>SPILGYWKIKGLVQPTRLLLEYLEEKYEEHLYERDEGDKWRNKKFELGLEFPNLPYYIDGDVKLTQSMAIIRYIADKHNMLGGCPKERAEISMLEGAVLDIRYGVSRIAYSKDFETLKVDFLSKLPEMLKMFEDRLCHKTYLNGDHVTHPDFMLYDALDVVLYMDPMCLDAFPKLVCFKKRIEAIPQIDKYLKSSKYIAWPLQG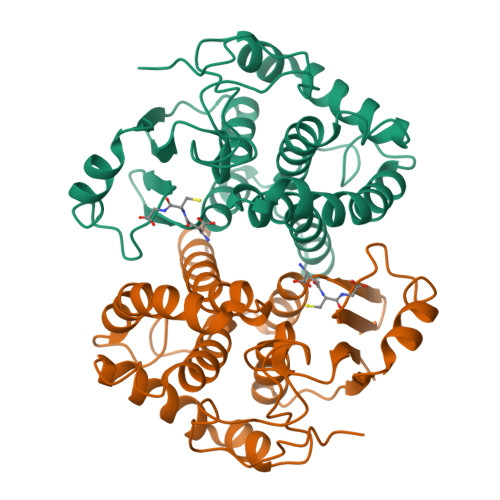WQATFGGGDHPPKSDPQQHHLGGAKQAGDV[2x]> VNGAGLLQTVWGPVCELTSELDGQAGAALKKEQEMLAKINDMQMAQLRAAIYL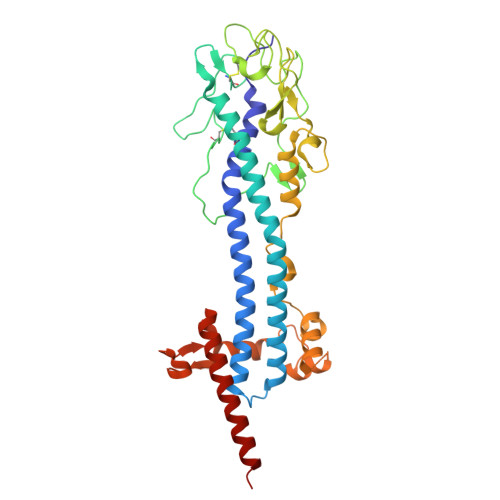AKNPSTPHQNALAVLTAYYAERAGSGKAYFLHALPKAVDSIRRAAYLKGHLDEYLNLLEKSSGGNNKCLVTTDDATVATRGGDQKLAGKNCKLSLSPLKPVDAALTYITKAGVGKLRYDDGGAGGNAVTPSKSGVHACKLLIAHNTAGYGDGGGVTADIDVFAGYMKVKATDAEPKLAAKSDLEEGGGGGAEAWKALHTAIKQEADAEAAELTNETGKLGERRHFLAAATNVLGTGAAGTGNAGRAAVEAAFGSDSEGGDRKIIELIEKELIVKGTANRDADESLGNIKTLKELGELLSYFQLKNSNTINELRNKLKAV>MGSIGSMGKPIEGFLVAAIQFPVPIVNSRKDIDHNIESIIRTLHATKAGYPGVELIIFPEYSTQGLNTAKWLSEEFLLDVPGKETELYAKACKEAKVYGVFSIMERNPDSNKNPYNTAIIIDPQGEIILKYRKLFPWNPIEPWYPGDLGMPVCEGPGGSKLAVCICHDGMIPELAREAAYKGCNVYIRISGYSTQVNDQWILTNRSNAWHNLMYTVSVNLAGYDNVFYYFGEGQICNFDGTTLVQGHRNPWEIVTGEIYPKMADNARLSWG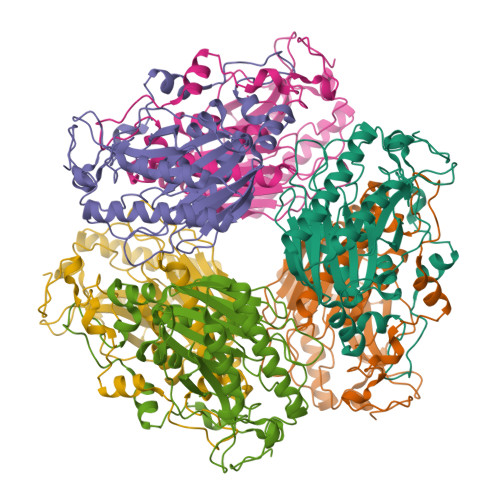LENNIYNLGHRGYVAKPGGEHDAGLTYIKDLAAGKYKLPWEDHMKIKDGSIYGYPTTGGRFGK[2x]>[2x]MIE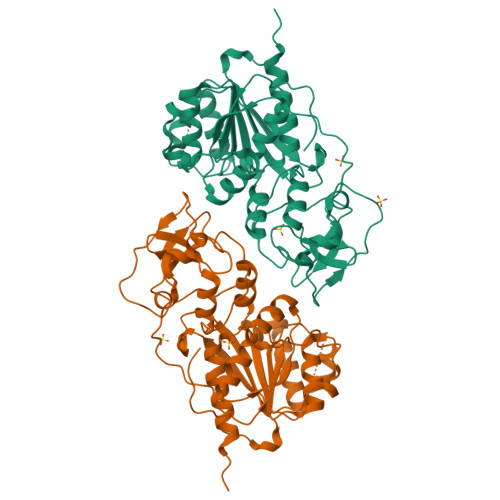IKDKQLTGLRFIDLFAGLGGFRLALESCGAECVYSNEWDKYAQEVYEMNFGEKPEGDITQVNEKTIPDHDILCAGFPCQAFSISGKQKGFEDSRGTLFFDIARIVREKKPKVVFMENVKNFASHDNGNTLEVVKNTMNELDYSFHAKVLNALDYGIPQKRERIYMICFRNDLNIQNFQFPKPFELNTFVKDLLLPDSEVEHLVIDRKDLVMTNQEIEQTTPKTVRLGIVGKGGQGERIYSTRGIAITLSAYGGGIFAKTGGYLVNGKTRKLHPRECARVMGYPDSYKVHPSTSQAYKQFGNSVVINVLQYIAYNIGSSLNFKPY We report biochemical properties and crystal structures of the LD-carboxypeptidases LdcB from Streptococcus pneumoniae, Bacillus anthracis, and Bacillus subtilis. The enzymes are active against bacterial cell wall tetrapeptides and adopt a zinc-carboxypeptidase fold characteristic of the LAS superfamily. LD-carboxypeptidases subsequently hydrolyze the L-Lys[A2pm]—D-Ala bond to release the tripeptide. The LdcB enzymes are single domain proteins comprising two subdomains separated by a V-shaped cleft.

The crystal structures of SpLdcB and Bacillus anthracis LdcB (BaLdcB) were solved by single wavelength anomalous dispersion (SAD); BsLdcB was solved by molecular replacement. Though the BaLdcB structure contains the same subdomain, it is less well structured in this region than BsLdcB and SpLdcB, and, as a consequence, the β1–β3 sheet is not formed. In SpLdcB, the liganding residues are His153, Asp160, and His207; the equivalents in BsLdcB/BaLdcB are His185/His160, Asp192/Asp167, and His244/His219. SpLdcB, BaLdcB, and BsLdcB share pairwise sequence identities of ∼30%, and they superimpose on ∼155 common Cα atoms with a root-mean-square deviation (rmsd) of 1.5 Å–1.8 Å. The active sites of SpLdcB, BaLdcB, and BsLdcB are, to all extents and purposes, indistinguishable. The cleft between subdomains is 15–18 Å wide at the top and 15 Å deep and narrows down to the base where a Zn2+ ion, added to the enzyme during purification, is located, which is coordinated in a tetrahedral manner by three amino acids.

>SNAASSFASVQAVVNKEYGLPEDYKPEDLVVPNVPFSFSGTLEKSYLRKEAAEALERLFDLANKEGIQLNAVSGFRSYDYQKKLYANNVKRKGQEHTDRFSAKPGHSEHQTGLTMDVSSKSANNELELTFANTKEGKWLKENAHRAGFIIRYPKGKESITGYAYEPWHIRYVGDIAESIYKKKLTLEEYMNL[2x]> GSSGSSGMQIGKIIKVSGPLVMAENMSEASIQDMCLVGDLGVIGEIIEMRQDVASIQVYEETSGIGPGEPVRSTGEALSVELGPGIISQMFDGIQRPLDTFMEVTQSNFLGRGVQLPALDHEKQWWFEATIEEGTEVSAGDIIGYVDETKIIQHKIMVPNGIKGTVQKIESGSFTIDDPICVIETEQGLKELTMMQKWPVRRGRPIKQKLNPDVPMITGQRVIDTFFPVTKGGAAAVPGPFGAGKTVVQHQIAKWSDVDLVVYVGCGERGNEMTDVVNEFPELIDPNTGESLMERTVLIANTSNMPVAAREASIYTGITIAEYFRDMGYDVAIMADSTSRWAEALREMSGRLEEMPGDEGYPAYLGSRLAEYYERSGRVIALGSDQREGSITAISAVSPSGGDISEPVTQNTLRVVKVFWGLDSSLAQKRHFPSINWIQSYSLYSTEVGRYMDQILQQDWSDMVTEGMRILQEEEQLNEIVRLVGIDSLSDNDRLTLEVAKSIREDYLQQNAFDDVDTFTSREKQFNMLKVILTFGKEARKALSLGAYFNEIMEGTVAVRERISRSKYIPEEELAKISSINEEIKETIQLIVSE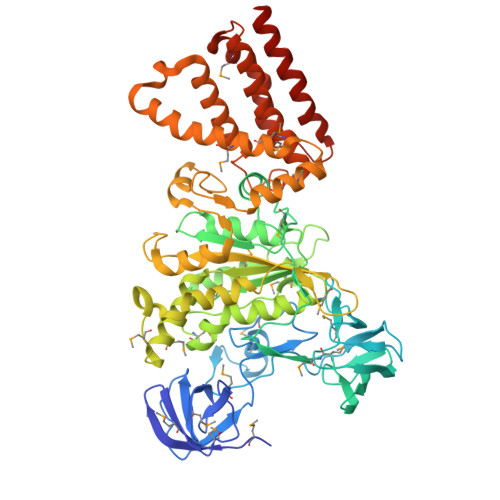GGMTDD>ASWSHPQFEKIEGRRDRGPEFMAKQYKNLVNGEWKLSENEITIYAPATGEELGSVPAMTQAEVDAVYASAKKALSDWRTLSYVERAAYLHKAADILVRDAEKIGAILSKEVAKGHKAAVSEVIRTAEIINYAAEEGLRMEGEVLEGGSFEAASKKKIAIVRREPVGLVLAISPFNYPVNLAGSKIAPALIAGNVVALKPPTQGSISGLLLAEAFAEAGIPAGVFNTITGRGSVIGDYIVEHEAVNFINFTGSTPIGEGIGKLAGMRPIMLELGGKDSAIVLEDADLALAAKNIVAGAFGYSGQRCTAVKRVLVMDKVADQLAAEIKTLVEKLSVGMPEDDADITPLIDTSAADFVEGLIKDATDKGATALTAFNREGNLISP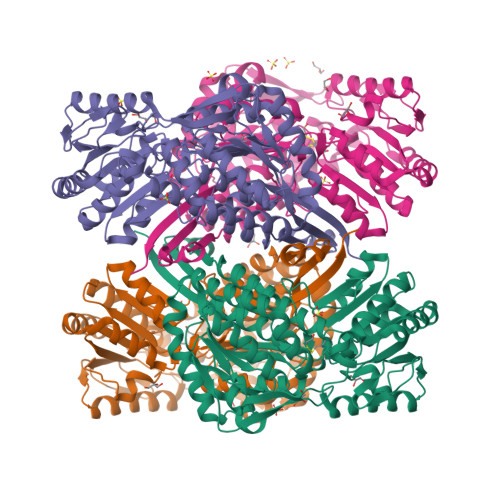VLFDHVTTDMRLAWEEPFGPVLPIIRVTTVEEAIKISNESEYGLQASIFTTNFPKAFGIAEQLEVGTVHLNNKTQRGTDNFPFLGAKKSGAGVQGVKYSIEAMTTVKSVVFDIQ[8x]2′,3′-cyclic nucleotide 3′-phosphodiesterase (CNPase) comprises 4% of total myelin protein in the central nervous system (CNS), being the most abundant CNS non-compact myelin protein4. CNPase consists of an N-terminal polynucleotide kinase-like domain10, a catalytic phosphodiesterase domain11, and a membrane-anchored C-terminal tail, which contains a cysteine residue that undergoes isoprenylation. The catalytic domain enables the rapid hydrolysis of nucleoside 2′,3′-cyclic phosphates to nucleoside 2′-phosphates. The CNPase catalytic site, lying in a groove between two lobes, has pseudo two-fold symmetry and contains two apposing His-X-Thr-X (X denotes a hydrophobic residue) motifs, characteristic for 2H phosphoesterases 113537.

Pro225 and Pro296 reside in loops α3-β2 and α6-β5, respectively, flanking the edges of the active site – Pro296 near the adenine moiety and Pro225 on the 5′-side of the ligand, next to Pro226. Interestingly, the mutant P296G has a marginally higher kcat than the wild-type enzyme. In P296G, which exhibits a higher kcat than wild-type CNPcat, while kcat/KM remains in similar range, the mutation-containing loop α6-β5 is disordered in the crystal structure, but adopts a different conformation compared to wild-type CNPcat. In the P296G structure, a 2′-AMP product is present in the active site. In contrast to the wild type enzyme, the adenine base is in a conformation similar to that seen in V321A before, and the β5-α7 loop has similarly adopted the open state. The latter, together with earlier liganded structures with an open β5-α7 loop34, suggests that loop opening is not an artifact caused by the V321A mutation, but rather a stabilized state so far not seen in crystal structures of the wild-type protein in complex with 2′-AMP. Additionally, the activity is probably not hindered by the observed base-flipping phenomenon, as demonstrated by P296G. Furthermore Arg307 has moved slightly away from the active site to the general direction where Gln307 would reside in the R307Q structure and Arg307 in the sulphate complex38. This, again, suggests that active site loop dynamics are linked to the conformation of Arg307. On the other hand, some mutant variants, such as P296G, even appeared slightly more stable than the wild-type protein.

> GGLEKDFLPLYFGWFLTKKSSETLRKAGQVFLEELGNHKAFKKELRHFISGDEPKEKLELVSYFGKRPPGVLHCTTKFCDYGKAAGAEEYAQQEVVKRSYGKAFKLSISALFVTPKTAGAQVVLTDQELQLWPSDLDKGSASEGLPPGSRAHVTLGCAADVQPVQTGLDLLDILQQVKGGSQGEAVGELPRGKLYSLGKGRWMLSLTKKMEVKAIFTGYYG>[3x]MKKGTDLLKKGFAKMVKHGVVMDVTNVEQAQIAEEAGAVAVMALERVPADIRAAGGVARMSDPALIEEIMDAVSIPVMAKCRIGHTTEALVLEAIGVDMIDESEVLTQADPFFHIYKKKFNVPFVCGARNLGEAVRRIWEGAAMIRTKGEA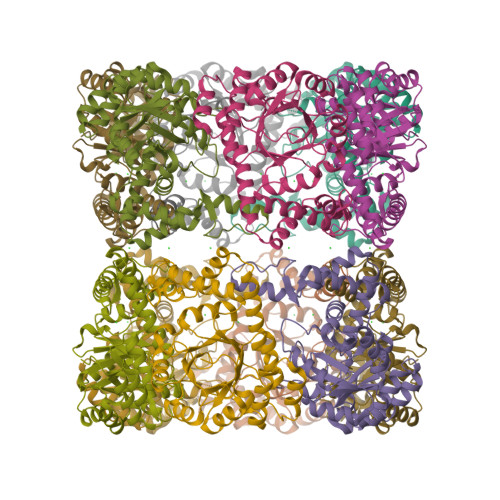GTGNIVEAVRHMRLMNEAIAQLQRMTDEEVYGVAKFYANRYAELAKTVREGMGLPATVLENEPIYEGFTLAEIIDGLYEVLLEVKKLGRLPVVNFAAGGVATPADAALMMQLGSDGVFVGSGIFKSENPLERARAIVEATYNYDKPDIVAEVSKNLGEAMKGIDITQISEAEKMQYRGD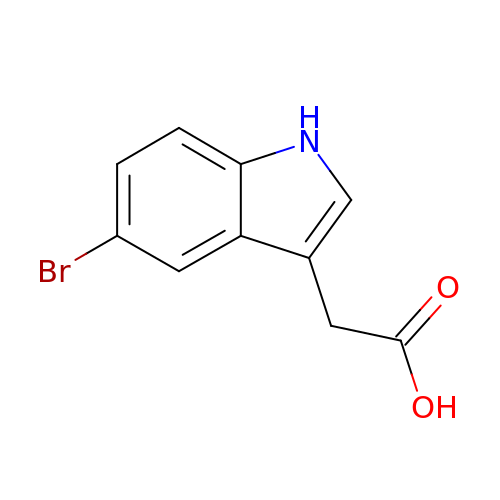(5-bromo-1H-indol-3-yl)acetic acid | C10 H8 Br N O2 | WTFGHMZUJMRWBK-UHFFFAOYSA-N>[4x]QTLLRNFGNVYD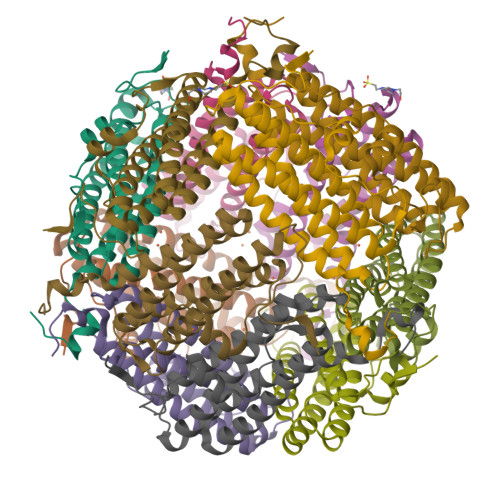NPVLLDRSVTAPVTEGFNVVLASFQALYLQYQKHHFVVEGSEFYSLHEFFNESYNQVQDHIHEIGERLDGLGGVPVATFSKLAELTCFEQESEGVYSSRQMVENDLAAEQAIIGVIRRQAAQAESLGDRGTRYLYEKILLKTEERAYHLSHFLAKDSLTLGFVQAA>GMVGINTDTENISELLKTYWSIQRISAGYADQNAASLGLTIQQLAMINVIYSTPGISVA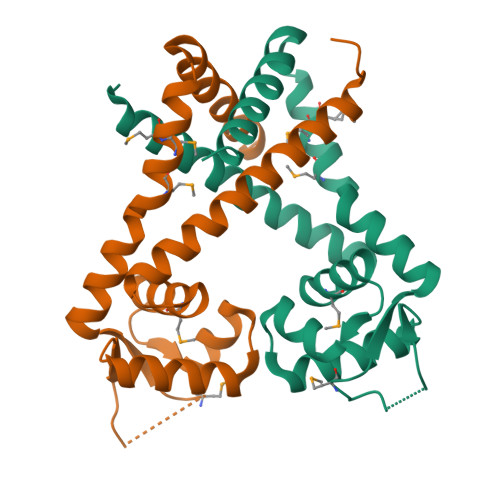DLTKRLIITGSSAAANVDGLISLGLVVKLNKTIPNDSMDLTLKLSKKGEDLSKRSTANAFMYKAMMKVFENLTENEIEELIRLNKKVETLLKKSK[8x]tert-butyl 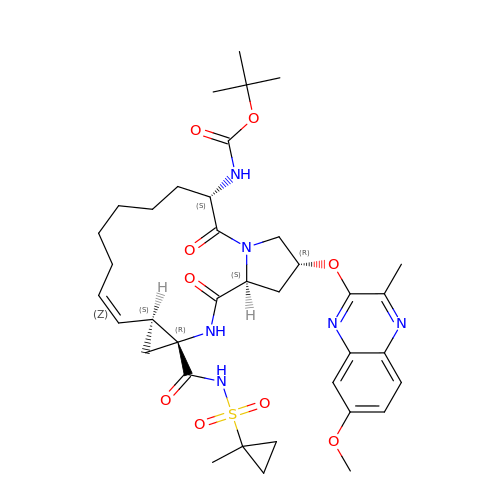[(2R,6S,12Z,13aS,14aR,16aS)-2-[(7-methoxy-3-methylquinoxalin-2-yl)oxy]-14a-{[(1-methylcyclopropyl)sulfonyl]carbamoyl}-5,16-dioxo-1,2,3,5,6,7,8,9,10,11,13a,14,14a,15,16,16a-hexadecahydrocyclopropa[e]pyrrolo[1,2-a][1,4]diazacyclopentadecin-6-yl]carbamate | C37 H50 N6 O9 S | OCYIAXNHVLIDIT-IIVIQOIMSA-N>[2x]APTAPSIDMYGSNNLQFSKIELAMETTSGYNDMVKYHELAKIKVKFNQWSGTSGDTYNVYFDGVKVATGAITGSQTTASFEYGQGGLYQMEIEACDATGCSKSAPVEITIADTDGSHLKPLTMNVDPNNKSYNTDPSIVMGTYFVEWGIYGRDYTVDNMPVDNLTHILYGFIPICGPNESVKSVGGNSFNALQTACRGVNDYEVVIHDPWAAYQKSFPQAGHEYSTPIKGNYAMLMALKQRNPDLKIIPSIGGWTLSDPF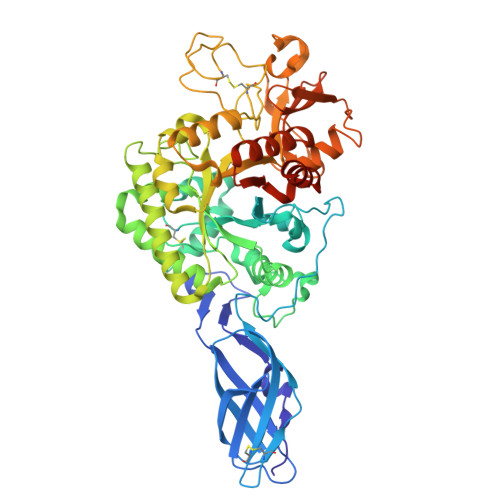YDFVDKKNRDTFVASVKKFLKTWKFYDGVDIDWEFPGGGGAAADKGDPVNDGPAYIALMRELRVMLDELEAETGRTYELTSAIGVGYDKIEDVDYADAVQYMDYIFAMTYDFYGGWNNVPGHQTALYCGSFMRPGQCDGGGVDENGEPYKGPAYTADNGIQLLLAQGVPANKLVLGTAMYGRGWEGVTPDTLTDPNDPMTGTATGKLKGSTAQGVWEDGVIDYKGIKSFMLGANNTGINGFEYGYDAQAEAPWVWNRSTGELITFDDHRSVLAKGNYAKSLGLAGLFSWEIDADNGDILNAMHEGMAGGVVTPPNRRSHHHHHH>[4x]AKGNDSKDFNNSYGISHITRDNMVKIPQQQNSDQFKVPAFDESTIKNIASAKGKNASGNTIDLDVWDSWPLQNADGTVATYHGYQIVFALAGDPKDSN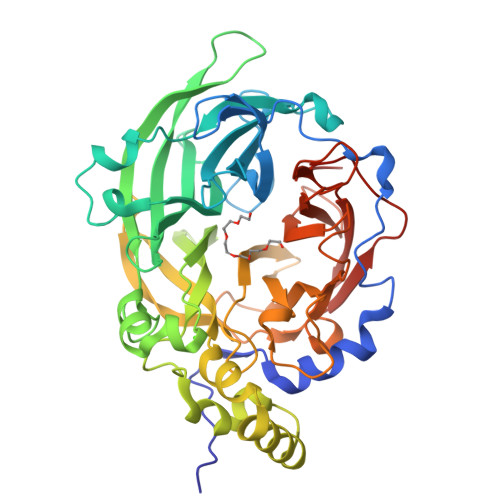DTSVYLFYKKAGDKSIDSWKNAGRVFKDSDKFVPNDPHLKNQTQEWSGSGTLTKDGKVRLFYTDYSGKQYGKQTLTTAQVNMSQPNDNTLKVDGVEDYKSIFDGDGKIYQTVQQFIDEGGYDTGDAHTLRDPHYIEDNGHKYLVFEANTGTEDGYQGEDSLYNRAYYGGNNPFFQSEKKKLLEGSNKEKASLANGALGIIELNDDYTLKKVMKPLITSNTVTDEIERANIFKKDGKWYLFTDSRGSKMTIDGIGQDDVYMLGYVSNTLTGKYKPLNDTGLVLHMDLDPNDKTFTYSHFAVPQTKGDNVVITSYMTNRGFYEDNHSTFAPSFLVNIDGSKTSVVKDRVLEQGQLTVDED>[2x]GPMRRSYEGYKVYGIVPESPDEAEILYQIRQSNPDLDFWHLTKQPGDEARVLVAPKDQRSFLIKLIRHGLHYQEVISDVEGTLAPYNEPRTRGMSLDR;>[2x]DVSTSYLRHNEINEYLQTLSQKYPSLVSVEEAGTSYEGRSIKTITINKKPGNAVVFLDAGIHAREWIAPATALYAIEQLVEHSSENQEVLSNLTWVIMPVVNPDGYEFSHETDRFWRKT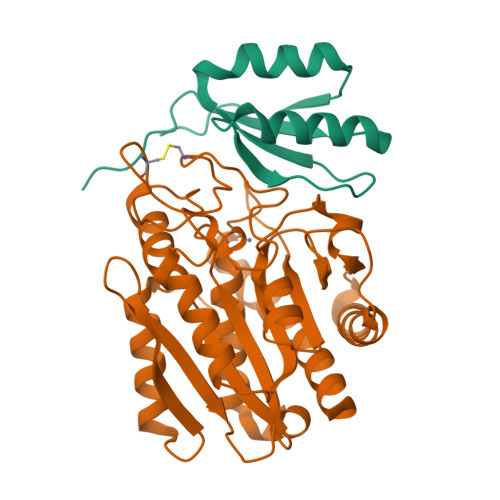RKPTGKSCKGTDGNRNFDYHWGEVGASTQACADTFRGETAFSEPETRAVRDAVMKLKGSCKFYLSLHSYGNYILYPWGWTSKLPETWEAIDEVAQAGAEAIKQSTGSRYTVGSSTNVLYAAAGGSDDWAFAVAEVPISITMELPGGGNGGFNPPPSSIEKIVNESWVGIKAMALKVAQMF>PQVKIYGLDSHLNPQKVRLSEVIHRCVVEALQFPKNKRF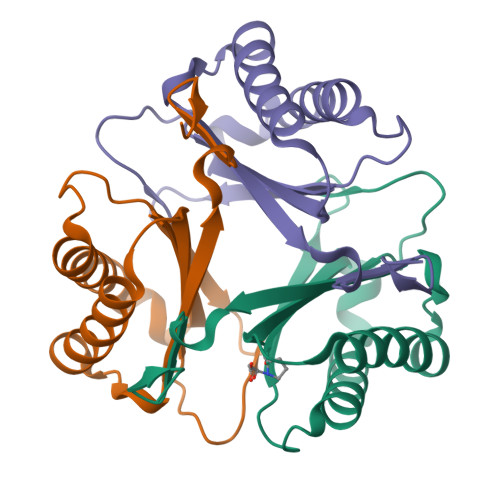HRFFPMKAEDMLFSEDRSSAYTIIEITMMEGRSKEAKKKLIALLFKHIEEELGIAGNDLEIFIQEAPAYHFGFRGMGGDEIVLDYKVEV[6x]>[2x]MKKLTFEIRSPAHQQNAIHAVQQILPDPTKPIVVTIQE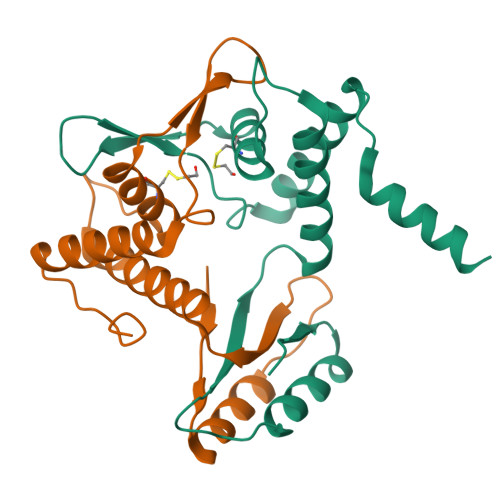RNRSLDQNRKLWACLGDVSRQVEWHGRWLDAESWKCVFTAALKQQDVVPNLAGNGFVVIGQSTSRMRVGEFAELLELIQAFGTERGVKWSDEARLALEWKARWGDRAA>[3x]MDKRVAEVAGAIVEAVRKILLDKRVTEAEYRAGVDYLTEVAQTRETALLLDVF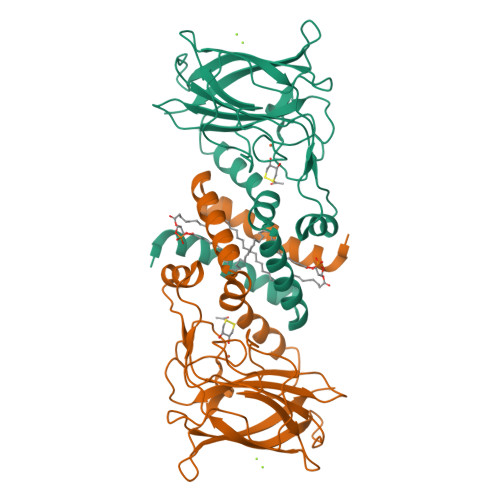LNSTIIEGKAQRSRTSAPAIQGPYFLEGAPVVEGVLKTYDTDDHKPLIIRGTVRSDTGELLAGAVIDVWHSTPDGLYSGIHDNIPVDYYRGKLVTDSQGNYRVRTTMPVPYQIPYEGPTGRLLGHLGSHTWRPAHVHFKVRKDGFEPLTTQYYFEGGKWVDDDCCHGVTPDLITPETIEDGVRVMTLDFVIEREQAEQRKSATETVA5-(propan-2-yl)-3-[(2S)-pyrrolidin-2-yl]-1,2,4-oxadiazole | C9 H15 N3 O | 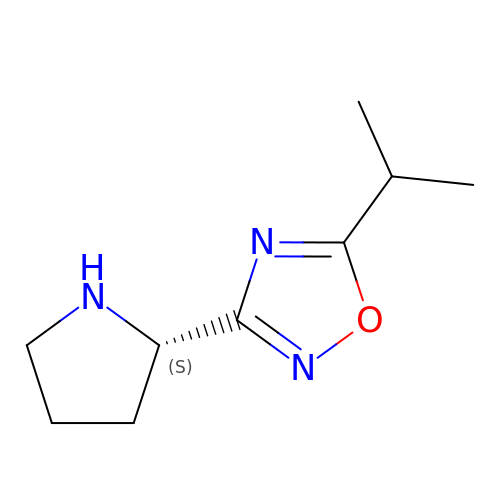WKTDGUSTKNDUEI-ZETCQYMHSA-N6-(5-methyl-1H-pyrazol-4-yl)-2-[(pyrrolidin-1-yl)methyl]thieno[3,2-d]pyrimidin-4(3H)-one 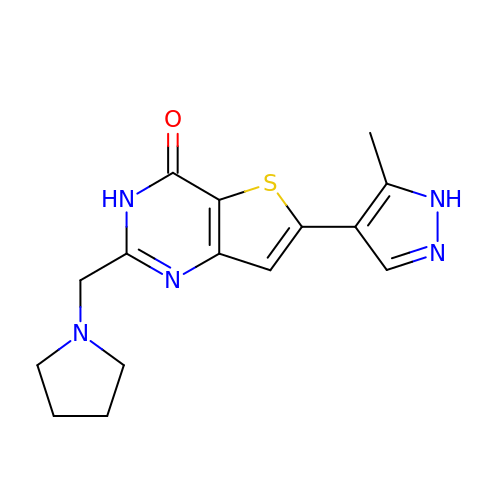| C15 H17 N5 O S | MUYIKPWUBQUQAV-UHFFFAOYSA-N>MSLDALELHRFLKGKIRTALPVEKVDRETLSLLYTPGVADVARACAEDPEKTYVYTSRWNTVAVVSDGSAVLGLGNIGPYGALPVMEGKAFLFKAFADIDAFPICLSESEEEKIISIVKSLEPSFGGINLEDIGAPKCFRILQRLSEEMNIPVFHDDQQGTAVVVSAAFLNALKLTEKKIEEVKVVVNGIGAAGYNIVKFLLDLGVKNVVAVDRKGILNENDPETCLNEY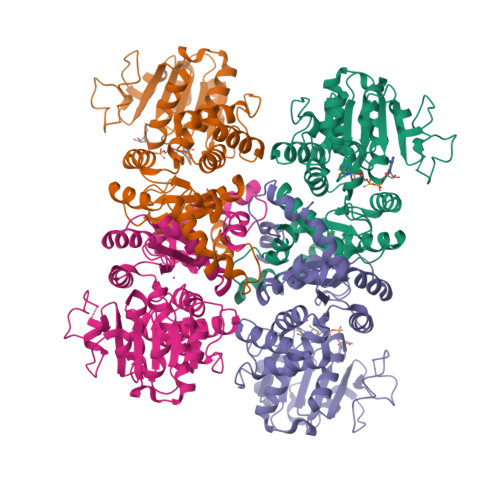HLEIARITNPERLSGDLETALEGADFFIGVSRGNILKPEWIKKMSRKPVIFALANPVPEIDPELAREAGAFIVATGRSDHPNQVNNLLAFPGIMKGAVEKRSKITKNMLLSAVEAIARSCEPEPERIIPEAFDMKVHLNVYTAVKGSAEGHHHHHH[4x]>MSNGILSQSIANMQQAEATIQSFSGLPQNAVNIQQNVGEVVAALLPQVQTMQQQVLAFAARLELQLTQQLANTGPFNPEALKAFVDLVQQEIAPIQTLTAQTLTASQSANDRITQDNIALQRIGVELQATIAGLQSNLDGARQELDSLNKKKLYLLGLGLLGLPGLIALAVTLTQTQNKVSSLEGQVNQIEGQIQRQQGFLGQTTAFSQQFGSLIDRVSKVGNTISLLGGDIANVARDAGQGDPELARLFFTAALTEVRTLQVDASLEHHHHHH[2x]

We show that the orthologue identified in A. hydrophila (AhlABC) is a haemolytic tripartite α-PFT, requiring all three components for maximal lysis, and we present the structures of the soluble forms of monomeric AhlB and tetrameric AhlC and the decameric pore form of AhlB. AhlC provides the initial single leaflet insertion, assembly with AhlB then producing an oligomeric hydrophobic pore, and finally recruitment of AhlA produces a hydrophilic fully active AhlABC pore. Structural and sequence analysis suggests this method of pore assembly may well occur throughout the tripartite α-PFT family.

As we have shown that the binary complex of AhlB and AhlC is partially haemolytic, the structure of the soluble form of AhlC was determined to 2.8 Å resolution in space group P6522 using Se-Methionine SAD, and refined to higher resolution (2.35 Å) using native data. Each subunit of AhlC had a very similar structure to that of the Type 2 conformation of the AhlB pore structure, (rmsd 2.4 Å), with a bundle of five α-helices forming the tail and helices α3 and α4 running the entire length of the protein and extending from the tail by 50 Å to form the neck and head domains. A stretch of 16 residues (L155-V171) at the end of α3 and the start of α4 in the head domain are hydrophobic, clearly indicating a possible method of membrane attachment. However, these sections of the two helices only extend over 15 Å, sufficient to span just one leaflet of the membrane, unlike AhlB where the hydrophobic parts of the equivalent structural elements can span the whole bilayer. Within the tetrameric assembly of soluble AhlC residues L156, L158, L160 and L163 in the α3–α4 hydrophobic head of subunit P pack against the hydrophobic residues L246 and L249 in the tails of both subunit Q and the symmetry related subunit P’, to form leucine zippers in the head to tail arrangement of the tetramer. Y154 of subunit P also forms π-stacking interactions with F250 in P’, and K152 of subunit P forms an ionic interaction with E257 of chain Q. The head of subunit P’ adopts the equivalent interactions in the tetramer. The other two hydrophobic heads from subunits Q and Q’ are more exposed on the tetramer surface and in the crystal pack against neighbouring hydrophobic heads from symmetry related tetramers. Thus, AhlC appears to use assembly of the quaternary structure to hide its hydrophobic head from the cytosol, rather than the conformational change mechanism seen in AhlB. Alignment of AhlC with YaxA or XaxA in their respective pores show that AhlC is closely related to both these structures, but that the extended conformation of AhlC subunit Q is more similar to YaxA or XaxA than that of AhlC subunit P, where the head is buried within the tetramer (rmsd 2.8 and 2.7 Å; and 4.0 and 2.8 Å, for subunits Q and P against YaxA and XaxA, respectively, Fig. 5c).> MYTNSDFVVIKALEDGVNVIGLTRGADTRFH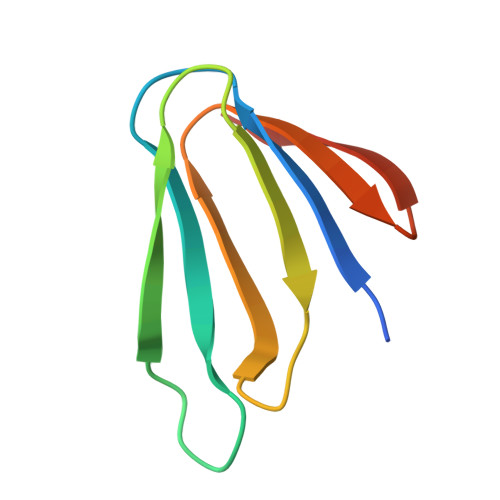HSEKLDKGEVLIAQFTEHTSAIKVRGKAYIQTRHGVIESEGKK> KENALL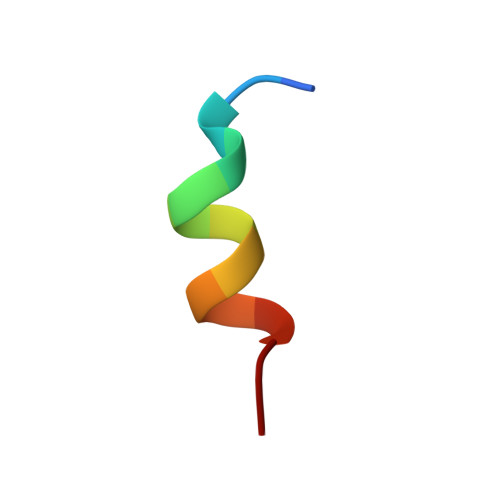RYLLDKD> MTSLFEPAQAGDIALANRIVMAPLTRNRSPGAIPNNLNATYYEQRATAGLIVTEGTPISQQGQGYADVPGLYKREAIEGWKKITDGVHSAGGKIVAQIWHVGRISHTSLQPHGGQPVAPSAITAKSKTYIINDDGTGAFAETSEPRALTIDDIGLILEDYRSGARAALEAGFDGVEIHAANGYLIEQFLKSSTNQRTDDYGGSIENRARFLLEVVDAVAEEIGAGRTGIRLSPVTPANDIFEADPQPLYNYVVEQLGKRNLAFIHVVEGATGGPRDFKQGDKPFDYASFKAAYRNAGGKGLWIANNGYDRQSAIEAVESGKVDAVAFGKAFIANPDLVRRLKNDAPLNAPNQPTFYGGGAEGYTDYPALAQHHHHHH

We determined the crystal structure of the enzyme NerA, which has been shown to exhibit dual ene-reductase and nitro-reductase activity with α,β-unsaturated nitro compounds, from A. radiobacter. NerA exhibits a TIM-barrel fold typical for OYE-like proteins, and all catalytically important active site residues are conserved. Residues stabilizing the electron-withdrawing group (EWG; e.g., carbonyl, carboxylic acid, nitro) of a ligand in an ene-reductase-like reaction are a histidine/asparagine pair (H178 and N181). The putative proton donor residue is Y183.

The structures of NerA in complexation with 4-hydroxybenzaldehyde and with 1-nitro-2-phenylpropene were determined at 2.3 and 2.5 Å resolutions from orthorhombic crystals (space group P212121). The previously determined apo structure was used as the search model for molecular replacement. Both soaking structures had one molecule present in the asymmetric unit. The overall B factors were higher than in the apo structure, and the overall structures were identical to the apo one. Like in the apo structure, weaker density was observed for the loop β3 region in both complex structures. The electron density for the soaked inhibitor 4-hydroxybenzaldehyde allowed fitting of the compound with the aromatic ring placed parallel to the si-face of the FMN isoalloxazine ring and the hydroxy moiety bound between residues H178 and N181. The aldehyde moiety, on the other hand, was fitted in the space between the aromatic residues Y65 and Y356. Soaking experiments resulted in two complex structures of the enzyme: one with 4-hydroxybenzaldehyde and one with 1-nitro-2-phenylpropene. Both compounds were found to exhibit typical OYE binding modes to NerA.>GSHMSTLKEVQDNITLHEQRLVTTRQKLKDAERAVELDPDDVNKSTLQSRRAAVSALETKLGELKRELADLIAAQKLASKPVDPTGIE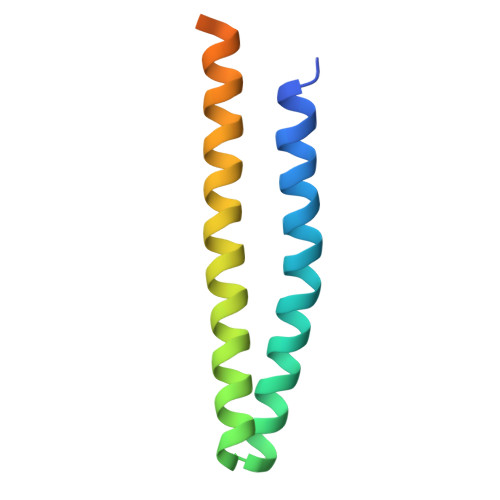PDDHLKEK[2x]> MVDQAVLDKLEAGYQKLQASADCHSLLKKYLTRQVLDACKNRKTQMGATLLDVVQSGFENLDSGVGLYAPDAESYTLFKELFDPVIDDYHKGFKPTDKHPPTDFGDVNTLCNVDPDNQFVISTRVRCGRSLQGYPFNPCLTEAQYKEMEDKVKGQLNSFEGE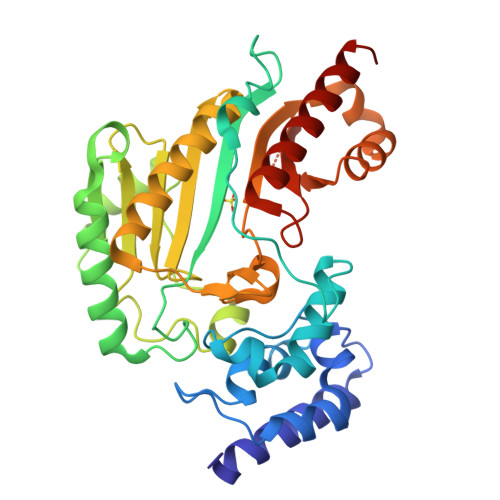LKGTYYPLLGMDKATQQQLIDDHFLFKEGDRFLQAANACRYWPVGRGIFHNDNKTFLIWCNEEDHLRIISMQKGGDLKQVFSRLINGVNHIEKKLPFSRDDRLGFLTFCPTNLGTTIRASVHIKLPKLAADRKKLEEIAGKYNLQVRGTAGEHTESVGGVYDISNKRRMGLTEYQAVKEMQDGILELIKIEKSM>[8x]GSHMSYNNIPAGKDAPNDIYVIIEIPANAAPIKYEIDKDSDALFVDRFMGTAMFYPANYGYVPNTLSEDGDPLDVLVVTPYPVAAGSVIRCRPVGKLNMEDDGGIDAKLIAVPHEKLSPLYKDVKEYTDLPQLLINQVEHFFSHYKDLEPGKWVKISGWEGADVAKAEVIKAIEAAK

However, because PPi is stable under normal conditions, inorganic pyrophosphatase (PPase) has evolved to specifically hydrolysis the molecule. Here, we solved four crystal structures of a family I type PPase from a strain of the pathogen Acinetobacter baumannii. The crystal structures of AbPPase showed that the enzyme has a typical Rossman fold domain that is highly conserved compared to other PPases. Family I PPases are hexamers formed by two stacks of trimers.

Structure 2 was solved from a crystal produced in the presence of Mg2+ and PPi. In this structure, three Mg2+ ions (M1, M2, and M3) and one PPi are bound to the catalytic center. Na+ was not detected in Structure 2. However, the space group of Structure 2 is H3 in which there are eight AbPPase monomers in the asymmetric unit. With this information, we set up the crystallization conditions to contain PPi and Mg2+ at a ratio of 5:1. This allowed us to then co-crystal AbPPase with PPi. By carefully analyzing Structure 2, we found that the electron density of eight AbPPase catalytic centers is different. Interestingly, electron density maps of the catalytic centers are different. This indicates that PPi in the AbPPase catalytic center can fluctuate and interact with different amino acid residues, Mg2+ and water molecules. In our structure, we found water (W2) 3.3 Å distant from pyrophosphate O3. W2 was not coordinated to any amino acid residue or divalent cation, suggesting that this water molecule directly comes from the solvent.Unique among viruses, some giant viruses utilize histones to organize their genomes into nucleosomes. Melbournevirus encodes a distinct H2B-H2A histone doublet variant in addition to the canonical H4-H3 and H2B-H2A doublets. This viral histone variant has a truncated H2B portion and its amino acid sequence deviates from that of the main viral H2B-H2A throughout the entire coding region.

To investigate whether the putative histone variant MV-varH2B-H2A can form viral NLPs with MV-H4-H3, we used our standard procedure to assemble nucleosomes with a 147 bp DNA fragment (Widom 601 positioning sequence). We were able to determine the structure of MV-varNLP to an overall resolution of 4.4 Å, with higher resolution observed for the protein core, while parts of the DNA and the tail regions are less well defined. MV-varNLP contains the requisite two copies of MV-H4-H3 and MV-varH2B-H2A (although one copy is better resolved than the other), and binds DNA in the canonical superhelical configuration typical for all nucleosomes. However, only about 90 bp of DNA are represented by density in MV-varNLP, compared to 124 bp in the MV-NLP density, and 147 bp in most canonical eukaryotic nucleosome structures. The H2B region of the variant histone doublet provides the requisite configuration for a stable four-helix bundle interface with the H4 portion of MV-H4-H3, and strong contacts with the DNA are established at this site (SHL ± 3.5). The MV-varH2B α3 helix is one turn shorter than in other H2B-like structures, and the adjacent αC helix, which defines the surface of the nucleosome, is two turns shorter than in any other H2B known to date. The connector between H2B and H2A is much shorter in the variant histone and fails to form the “knuckle domain” that in MV-H2B-H2A contact DNA at SHL 4.5. Due to its absence in MV-varH2B-H2A, no contacts with DNA are established at SHL 4.5, even though this region maintains an overall positively charged surface. Interestingly, a conserved cysteine in the MV-varH2A L1 loop forms a disulfide bond with the second varH2A, supported by well-defined electron density, seemingly stapling together the two MV-varH2B-H2A variant moieties. MV-varNLP (with a melting temperature of 49.5 ± 0.55 °C) is destabilized compared to MV-NLP (52.8 ± 0.4 °C), and this difference, although relatively modest, is statistically significant.

>[2x]MDRVGKYGLFIKRISPKDADITKESLETVNNMLVFLAEKLTKQANIIIDQKTLRHDAFLWLLTDIQGELGKHSQDFANSVLYGEKELVFPTKRTENLMRKNTCLRISQSAVKTLTAILEYFCGQIMEASFSQAKKSKRKRIRPIDIEAAISQDKELHSMFGKGVISGR;>[2x]MSKAGKKVKAQQHGHLADHVSVGETQIPKASTQHLLRKAGSLSAAGDTEVPIRGFVHMKLHKLVQKSLLAMQLAKRKTIMKSDVKKAAELMHLPVFAIPTKDSGAKGSVFLSCRQKGAGSAGTGSETNSQEVRSQMKSTCLIIPKERFRTMAKEISKKEGHDVHIAEAALDMLQVIVESCTVRLLEKALVITYSGKRTRVTSKDIETAFMLEHGPL>GSHMTPTPRPTDGVDIYFGMPGEISEHEGFLRAKMDLEERRMRQINEVMREWAMADNQSKNLPKADRQALNEHFQSILQTLEEQVSGERQRLVETHATRVIALINDQRRAALEGFLAALQADPPQAERVLLALRRYLRAEQKEQRHTLRHYQHVAAVDPEKAQQMRFQVHTHLQVIEERVNQSLGLLDQNPHLAQELRPQIQELLH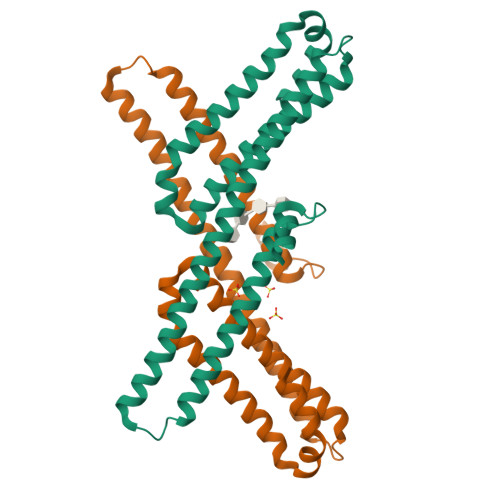SEHLGPSE[2x]>MAGKAHRLSAEERDQLLPNLRAVGWNELEGRDAIFKQFHFKDFNRAFGFMTRVALQAEKLDHHPEWFNVYNKVHITLSTHECAGLSERDIN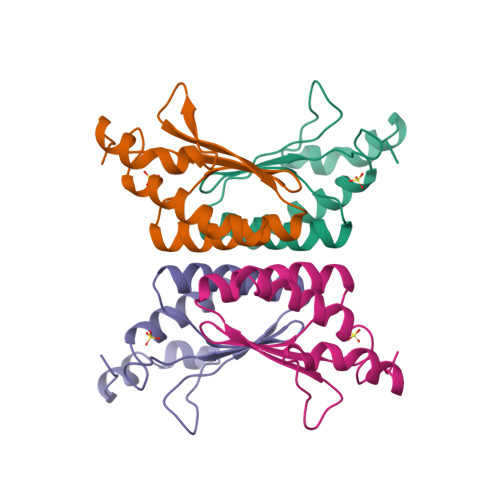LASFIEQVAVSMT[8x]N-[3-(4-{[(2-aminoethyl)(methyl)amino]methyl}-1H-pyrrol-3-yl)phenyl]propanamide 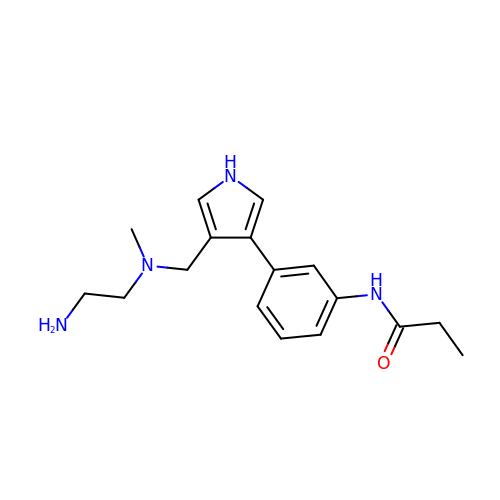| C17 H24 N4 O | ZXTYIIDDTFQCGV-UHFFFAOYSA-N>[4x]MQPLFTQERRIFHKKLLDGNILATNNRGVVSNADGSNTRSFNIAKGIADLLHSETVSERLPGQTSGNAFEAICSEFVQSAFEKLQHIRPGDWNVKQVGSRNRLEIARYQQYAHLTALAKAAEENPELAAALGSDYTITPDIIVTRNLIADAEINRNEFLVDENIATYASLRAGNGNMPLLHASISCKWTIRSDRAQNARSEGLNLVRNRKGR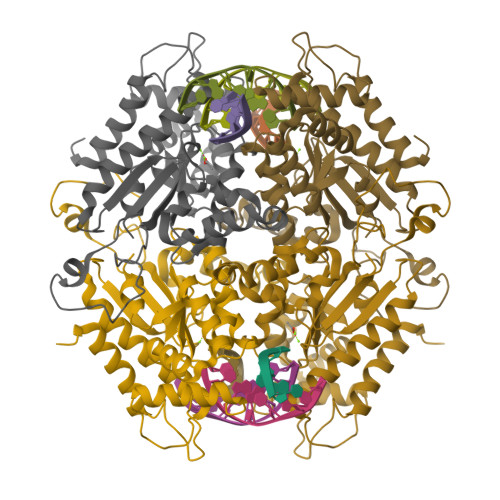LPHIVVVTAEPTPSRISSIALGTGEIDCVYHFALYELEQILQSLNYEDALDLFYIMVNGKRLKDISDLPLDLAV N-(3,3-diphenylpropyl)pyridine-3-carboxamide 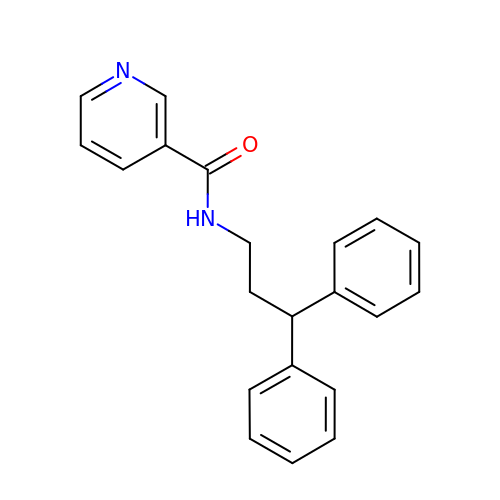| C21 H20 N2 O | GDHXZIQAOUBZCC-UHFFFAOYSA-N> MNSHPRLTPWKSSDEVVYLKGLFFPADREQISRDELYRQYEEAISLVEMYSSRTRVSHILQSTAHLFSALMMLESFEGGLDDTVRLTASMTIIRFVNGLLDPNQQSQFAIPLHLLAKKIDLPSLFVEFRHSATHDALPSLEMCKTCVDRAIDWVWDHYWDGVLSIVEPQVETDDLEESLIKELKDLFKQYRRIRRQNITKLYKFGDSTPEGKEYWTCIAGIKDHADMANFYNVMIERIVSNKLKWEHLRALFEPMMNHFIHLKGWDFPLGLIDSMLSKNYEYSKFRGIDDTERAYLNDQEFKCAQKWIRWLAIEQIDRYDDVLVS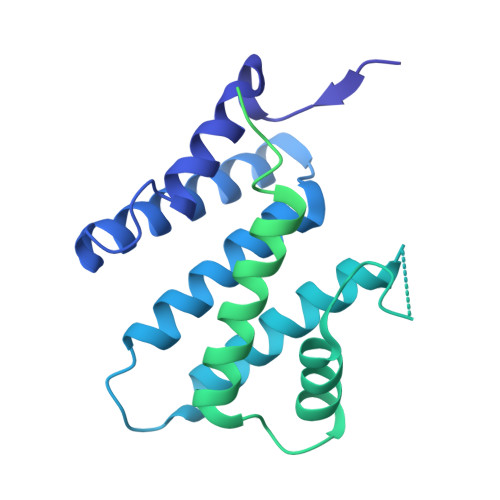KMIDTLGKTNHELNVELLEKLQSRFSADPVIKDKIQAKLTLIQRLSTDTKTKRMNNLEDIMSDLESLKKRAKVTPTLHIKSFESHPNWTPKPFGVI> MNLNIIMTVLPLLVSVAFL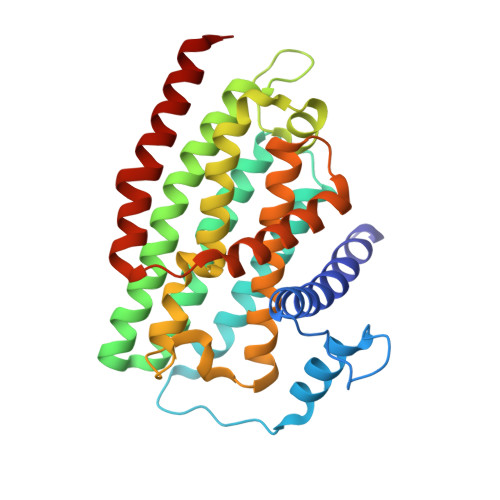TLSERAVMGSLQRRMGPAVSGAFGILQPFWDGFKLAVKEPILPANAAAGIFYAAPLICICICVASWCTLLLTDLSIGGLFLLLLSSLAVYGVLLAGYSCNSKYAFLGCLRSVSLMISYELVISVVILCVILETRDGNGFPCLNLTETASQTKIILIPAGLLFYICSLAESKRVPFDLPEAEAELVAGYNVEYSSLGFAVFFVAEYGNTLLMAALINIYFLGKLNSALIAAIFVSFIWVRGTLPRYRYDMFMQIGWKSLLPVALALYLAQASLGY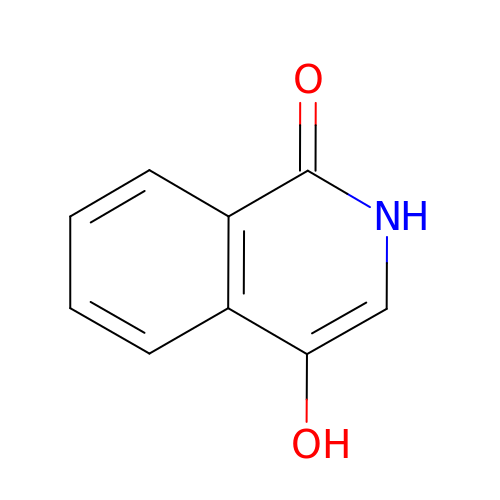4-oxidanyl-2~{H}-isoquinolin-1-one | C9 H7 N O2 | KOJRWXLHYKLCFJ-UHFFFAOYSA-N> MAETSEEVAVLVQRVVKDITNAFRRNPHIDEIGLIPCPEARYNRSPIVLVENKLGVESWCVKFLLPYVHNKLLLYRTRKQWLNRDELIDVTCTLLLLNPDFTTAWNVRKELILSGTLNPIKDLHLGKLALTKFPKSPETWIHRRWVLQQLIQETSLPSFVTKGNLGTIPTERAQRLIQEEMEVCGEAAGRYPSNYNAWSHRIWVLQHLAKLDVKILLDELSSTKHWASMHVSDHSGFHYRQFLLKSLISQTVIDSSVMEQNPLRSEPALVPPKDEEAAVSTEEPRINLPHLLEEEVEFSTDLIDSYPGHETLWCHRRHIFYLQHHLNGRFPHSMTQLSPADSPGGTLSDLHLIPAGSQLSQAMEVD;> GPLGSMGTPQKDVIIKSDAPDTLLLEKHADYIASYGSKKDDYEYCMSEYLRMSGIYWGLTVMDLMGQLHRMNREEILAFIKSCQHECGGISASIGHDPHLLYTLSAVQILTLYDSINVIDVNKVVEYVKGLQKEDGSFAGDIWGEIDTRFSFCAVATLALLGKLDAINVEKAIEFVLSCMNFDGGFGCRPGSESHAG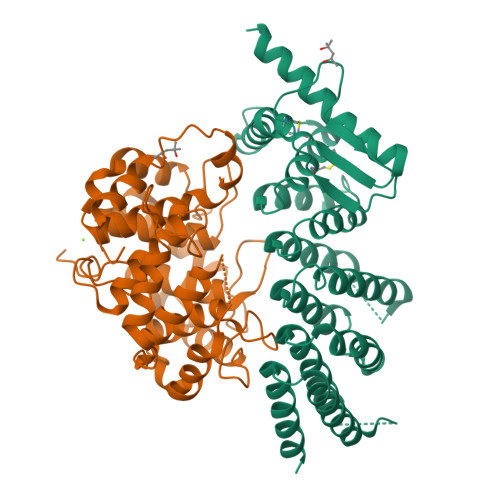QIYCCTGFLAITSQLHQVNSDLLGWWLCERQLPSGGLNGRPEKLPDVCYSWWVLASLKIIGRLHWIDREKLRNFILACQDEETGGFADRPGDMVDPFHTLFGIAGLSLLGEEQIKPVNPVFCMPEEVLQRVNVQPELVS>[2x]SDVENF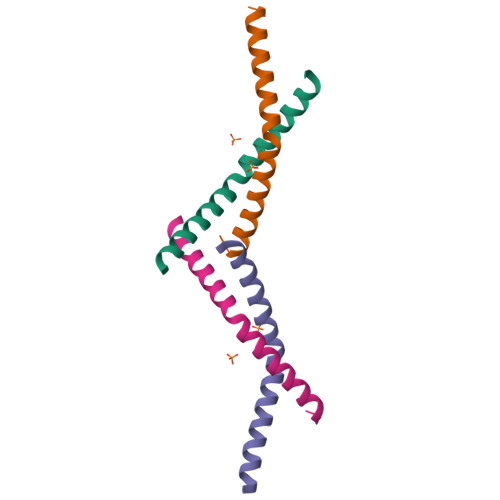ERLFSKLKEMKDKAATLPHEQRKVHAEKVAKAFWMAIGG>[4x]AMSLNIITVTLNMEKYNFL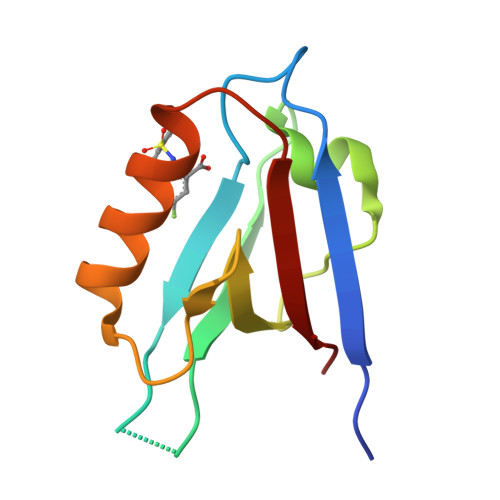GISIVGQSNERGDGGIYIGSIMKGGAVAADGRIEPGDMLLQVNEINFENMSNDDAVRVLREIVHKPGPITLTVAKS> MDMHMIVKVVAILAVLFLVYKLWESMNKPNASPLKIQNPYEKYMNSAEGGEYDAEDDDIYYPETDAEDDDIYTGETDDMYDGEDDDIYVQEGDDIEDAEDEPYDDSADMEQDVPKVQQPMMPLLTPSSQLLPKPSPEAADFAQFAPKNLQAQNFLTATQWIGVNTQGSSLKNANYDLRADPIIPKADVGPWMMSSVDPNIYQK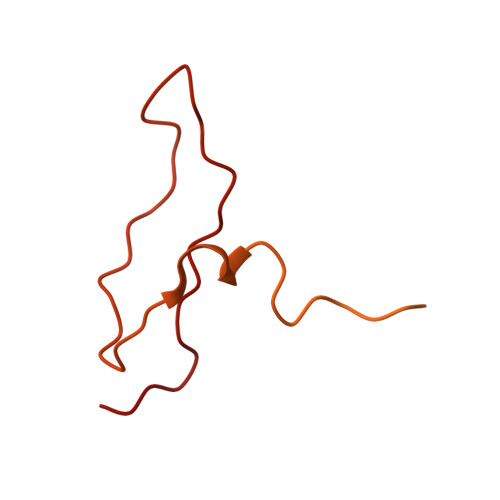PLFG>MMVAWWSLFLYGLQVAAPALAATPADWRSQSIYFLLTDRFARTDGSTTATCNTADQKYCGGTWQGIIDKLDYIQGMGFTAIWITPVTAQLPQTTAYGDAYHGYWQQDIYSLNENYGTADDLKALSSALHERGMYLMVDVVANHMGYDGAGSSVDYSVFKPFSSQDYFHPFCLIQNYEDQTQVEDCWLGDNTVSLPDLDTTKDVVKNEWYDWVGSLVSNYSIDGLRIDTVKHVQKDFWPGYNKAAGVYCIGEVLDGDPAYTCPYQNVMDGVLNYPIYYPLLNAFKSTSGSMDD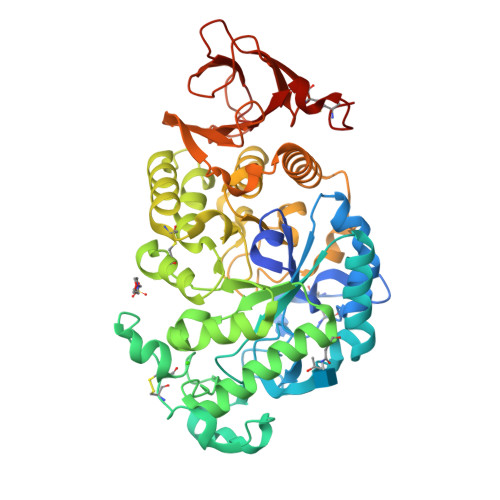LYNMINTVKSDCPDSTLLGTFVENHDNPRFASYTNDIALAKNVAAFIILNDGIPIIYAGQEQHYAGGNDPANREATWLSGYPTDSELYKLIASANAIRNYAISKDTGFVTYKNWPIYKDDTTIAMRKGTDGSQIVTILSNKGASGDSYTLSLSGAGYTAGQQLTEVIGCTTVTVGSDGNVPVPMAGGLPRVLYPTEKLAGSKICSSS[2x]> KWYYKTITFLPELCNNESLAAKCLRVLHGFNYQYETRNIGVSFPLWCDATVGKKISFVSKNKIELDLLLKQHYFVQMEQLQYFHISNTVLVPEDCTYVSFRR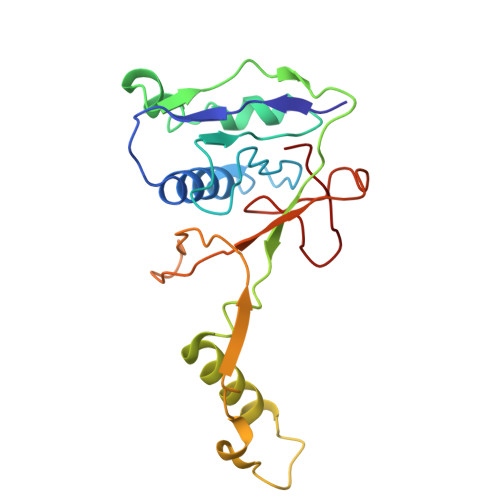CQSIDKLTAAGLARKIRRLEKRALSRGEAFDPSSFAQKEHTAIAHYHSLGESSKQTNRNFRLNIRMLSEQPREGNSIFSSYGLANSENSFQPVPL> MAHHHHATLTVPTTVPSVSEDCEQLRKAFSGWGTNEGLIIDILGHRNAEQRNLIRKTYAETYGEDLLKALDKELSNDFERLVLLWALDPAERDALLANEATKRWTSSNQVLMEIACTRSANQLLHARQAYHARYKKSLEEDVAHHTTGDFHKLLLPLVSSYRYEGEEVNMTLAKTEAKLLHEKISNKAYSDDDVIRVLATRSKAQINATLNHYKNEYGNDINKDLKADPKD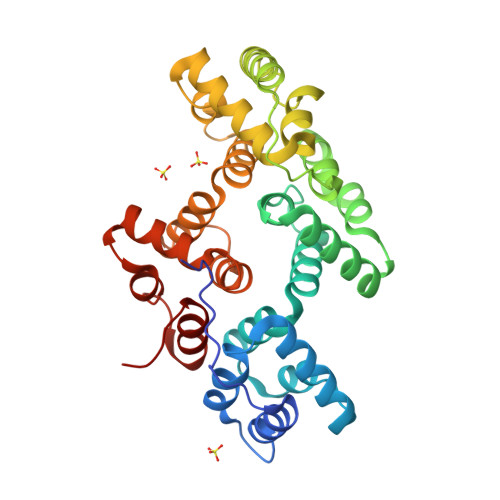EFLALLRSTVKCLVYPEKYFEKVLRLAINRRGTDEGALTRVVCTRAEVDLKVIADEYQRRNSVPLTRAIVKDTHGDYEKLLLVLAGHVEN> GPLGSDHDDSFHVILNKSSPEEQLGIKLVRRVDEPGVFIFNVLNGGVADRHGQL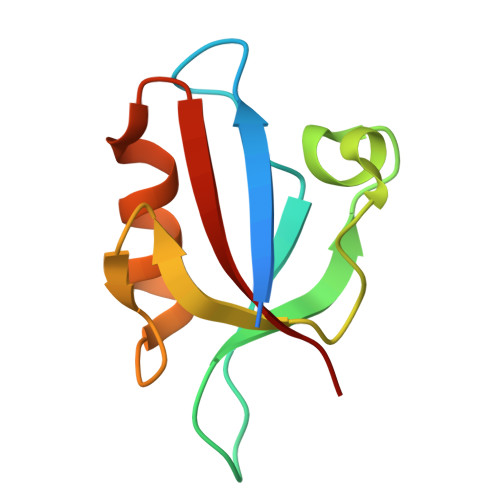EENDRVLAINGHDLRFGSPESAAHLIQASERRVHLVVSRQ>MRSRRVDVMDVMNRLILAMDLMNRDDALRVTGEVREYIDTVKIGYPLVLSEGMDIIAEFRKRFGCRIIADFKVADIPETNEKICRATFKAGADAIIVHGFPGADSVRACLNVAEEMGREVFLLTEMSHPGAEMFIQGAADEIARMGVDLGVK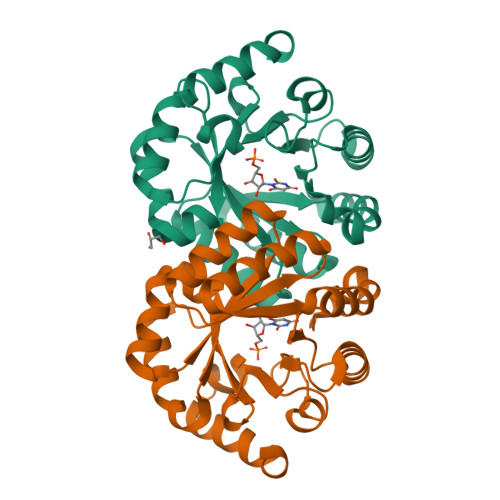NYVGPSVRPERLSRLREIIGQDSFLISPGAGAQGGDPGETLRFADAIIVGRSIFLADNPAAAAAGIIESIKDLLNP[2x]>[3x]VRSSSRTPSDKPVAHVVANPQAEGQLQWLNRRANALLANGVELRDNQLVVPSEGLYLIYSQVLFKGQGCPSTHVLLTHTIS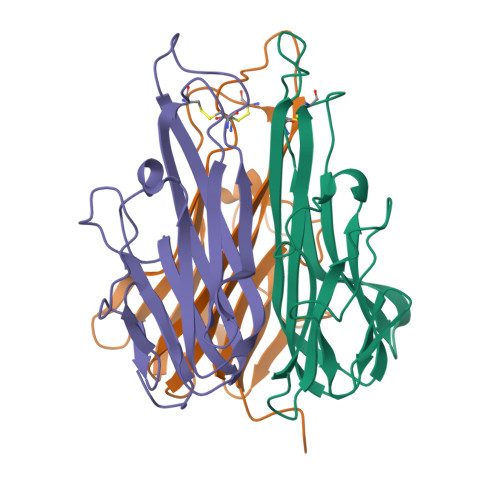RIAVSYQTKVNLLSAIKSPCQRETPEGAEAKPWYEPIYLGGVFQLEKGDRLSAEINRPDYLLFAESGQVYFGIIAL>MSGQGFRSILTGSFSTPCADNPTVAMVEAGYHHAGLDARYINCDVKASGLADAVKGAKAMEWVGFNCSLPHKVAVLDHLDDIAESARLIGAVNCVAIREGKLIGHNTDGKGFLASLKTVTSPAGKRVVILGAGGAARAIAVELALAGAAHITIVNRDASKA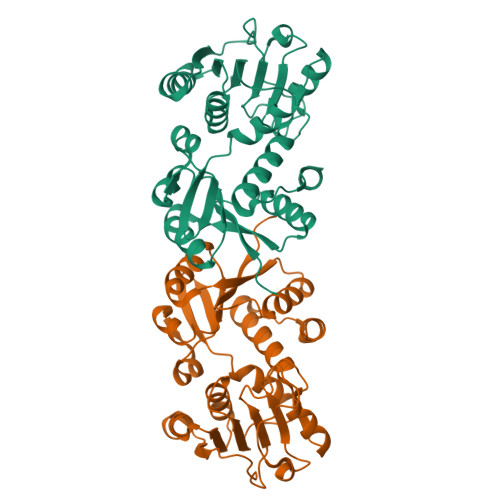ETIAALINDKTEATGEAQAWSGKFSLPTGTDILINATSIGLGDPNAAPPVEMGSLTKETVVADVIPNPPQTRFLKDAKALGCTTLDGLGMLVNQGVIGVEIWLGRTLDSAVMAQTLENIFGTENK[2x]> NYWYLQGLIHKQNGDLLQAAKCYEK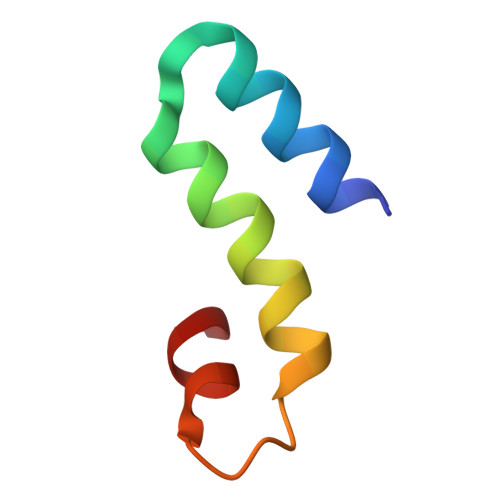ELGRLLRDAPSGIGSIFLS>[2x]MVMNLKQFSTYTQSRVDQYLEQQLSDYAPANQLHNAMRYSLFNGGKRIRPMLTYASAQLVGDISSLTDASAA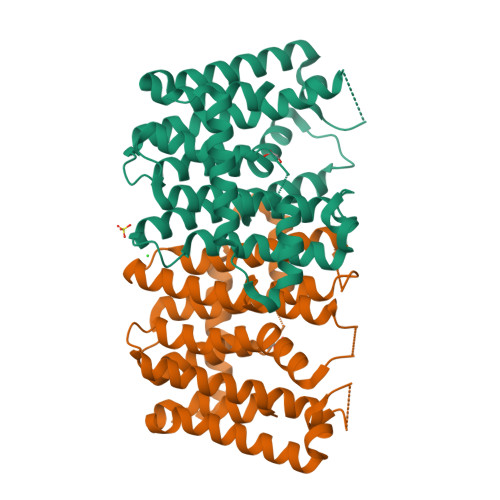ALESIHAYSLIHDDLPAMDNDELRRGKPTCHIQFDEATAILAGDALQTFAFELLSNPTSAQPELAIKLIQELVVASGRNGMITGQMIDLSSENKNISLAELEQMHVHKTGALIKASVRMGALSTGQVKPEQLAKLDAYAHAIGLAFQVQDDIIDLTSDTETLGKTQFSDAEANKATYPKLLGLDGAKALVVRLHEQAIAQISEFGDKSQPLTDLANYIIDRNHAENLYFQSHHHHHHWSHPQFEK>DGINQSGDKAGSTVYSAKGTSLEVGGRAEARLSLKDGKAQDNSRVRLNFLGKAEINDSLYGVGFYEGEFTTNDQGKNASNNSLDNRYTYAGIGGTYGEVTYGKNDGALGVITDFTDIMSYHGNTAAEKIAVADRVDNMLAYKGQFGDLGVKASYRFADRNAVDAMGNVVTETNAAKYSDNGEDGYSLSAIYTFGDTGFNVGAGYADQDDQNEYMLAASYRMENLYFAGLFTDGELAKDVDYTGYELAAGYKLGQAAFTATYNNAETAKK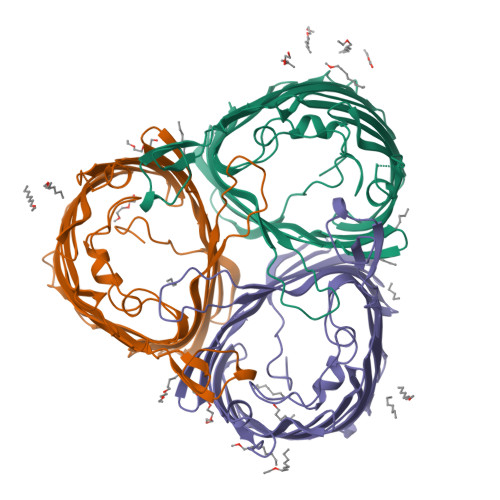TSADNFAIDATYYFKPNFRSYISYQFNLLDSDKASKVASEDELAIGLRYDF[3x]The ethylene-forming enzyme (EFE) is an Fe(II), 2-oxoglutarate (2OG), and l-arginine (l-Arg)-dependent oxygenase that either forms ethylene and three CO2/bicarbonate from 2OG or couples the decarboxylation of 2OG to C5 hydroxylation of l-Arg. l-Arg binds with C5 toward the metal center, causing 2OG to change from monodentate to chelate metal interaction and OD1 to OD2 switch of D191 metal coordination. The best characterized EFE is that from the Pseudomonas savastanoi (formerly Pseudomonas syringae) pv phaseolicola strain PK2, for which several crystal structures have been reported. This enzyme binds mononuclear Fe(II) using three side chains (H189, D191, and H268) with three water molecules completing the six-coordinate geometry. Here, we extend our understanding of EFE catalysis by carrying out biochemical, structural, and computational studies of the enzyme in complex with a substrate analogue and using two enzyme variants. In combination, the results presented here are compatible with the currently proposed enzyme mechanism,4−8 emphasize the necessity for OD2 of D191 to coordinate the metal, and highlight the importance of the second coordination sphere and longer range interactions in promoting EFE activity.

Third, we focused on the nearly inactive Y306A variant of the EFE for which the substitution occurs distant from the active site. We noted distinct behavior when investigating the MLCT transitions associated with Y306A EFE·Fe(II)·2OG and obtained insights from the structure of the Y306A EFE·Mn(II)·2OG complex that was crystallized in the presence of unbound l-Arg. Y306 is a generally conserved residue located 12 Å from the metal site, with the active site residue Y192 located in between. The substitution by alanine of Y306 in the EFE, a residue 12 Å away from the catalytic metal center, generates an interior cavity that leads to multiple local and distal structural changes that reduce l-Arg binding and significantly reduce the enzyme activity. Substitution of Y306 by alanine leads to a large conformational change of one loop with additional propagated changes to affect several residues important for l-Arg binding, accounting for the inactivity of this variant. UV–vis and structural studies both reveal that 2OG binds to the protein to yield a mixture of the monodentate- and bidentate-coordinated species. The loss of the MLCT transitions upon addition of l-Arg is consistent with a deficiency in l-Arg binding as revealed by its absence of this amino acid in the crystal structure despite being present in the crystallization buffer. In line with experimental studies, the binding energy calculated from the MD simulations using MMGBSA revealed a lower binding affinity of l-Arg in the Y306A variant enzyme.

> SHMTNLQTFELPTEVTGCAADISLGRALIQAWQKDGIFQIKTDSEQDRKTQEAMAASKQFCKEPLTFKSSCVSDLTYSGYVASGEEVTAGKPDFPEIFTVCKDLSVGDQRVKAGWPCHGPVPWPNNTYQKSMKTFMEELGLAGERLLKLTALGFELPINTFTDLTRDGWHHMRVLRFPPQTSTLSRGIGAHTDYGLLVIAAQDDVGGLYIRPPVEGEKRNRNWLPGESSAGMFEHDEPWTFVTPTPGVWTVFPGDILQFMTGGQLLSTPHKVKLNTRERFACAYFHEPNFEASAYPLFEPSANERIHAGEHFTNMFMRCYPDRITTQRINKENRLAHLEDLKKYSDTRATGS> MSQRIIQPSASDQQFPGKSDGYEYTVGPKQAITSEASTTYIPSRIYSESLLFKRQEASLSAMAFLFQEMISQLHRTCKTAGDFETKLSD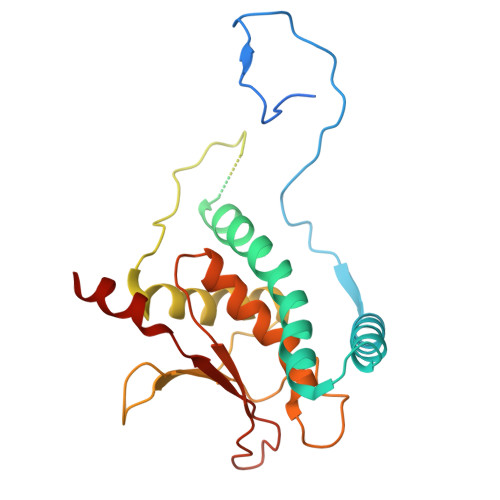YGHNIGIRLLELLNFRASSSPSSLPRASAFLSQNESSSKLSNASNSPGMLANSSTATSASANERLQEKQTESLSNYITKMRRRDLKILDILQFIHGTLWSYLFNHVSDDLVKSSERDNEYMIVDNFPTLTQFIPGENVSCEYFVCGIIKGFLFNAGFPCGVTAHRMPQGGHSQRTVYLIQFDRQVLDREGLRFG> MSNISRQAYADMFGPTVGDKVRLADTELWIEVEDDLTTYGEEVKFGGGKVIRDGMGQGQMLAADCVDLVLTNALIVDHWGIVKADIGVKDGRIFAIGKAGNPDIQPNVTIPIGAATEVIAAEGKIVTAGGIDTHIHWICPQQAEEALVSGVTTMVGGGTGPAAGTHATTCTPGPWYISRMLQAADSLPVNIGLLGKGNVSQPDALREQVAAGVIGLKIHEAWGATPAAIDCALTVADEMDIQVALHSDTLNESGFVEDTLAAIGGRTIHTFHTEGAGGGHAPDIITACAHPNILPSSTNPTLPYTLNTIDEHLDMLMVCHHLDPDIAEDVAFAESRIRRETIAAEDVLHDLGAFSLTSSDSQAMGRVGEVILRTWQVAHRMKVQRGALAEETGDNDNFRVKRYIAKYTINPALTHGIAHEVGSIEVGKLADLVVWSPAFFGVKPATVIKGGMIAIAPMGDINASIPTPQPVHYRPMFGALGSARHHCRLTFLSQAAAANGVAERLNLRS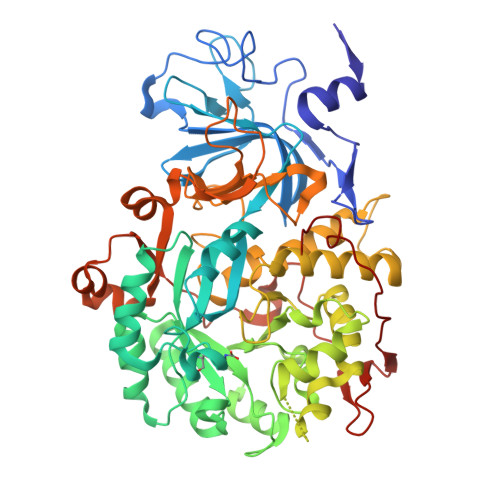AIAVVKGCRTVQKADMVHNSLQPNITVDAQTYEVRVDGELITSEPADVLPMAQRYFLF> SNARAIARPTRSEYLARINEENRLKHEIQELTQALALEKQNTVTLVAQAQQQAKAKPIVRSQPEKSLESTDQNTLALNIQFYDPKQLLSSVNQSVSVPYFKLCQLFLNKSIELCTKHYHLKATDIDVVDEFHAE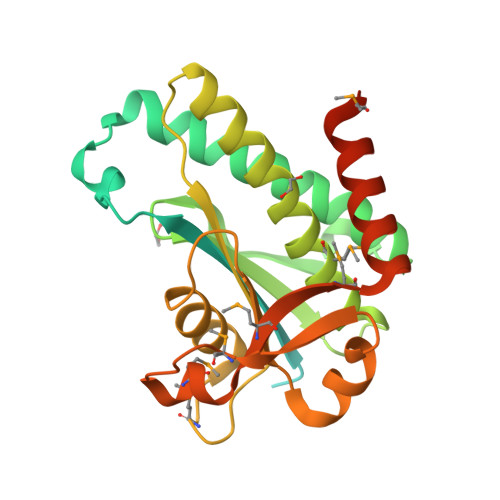GATLAISTSHPHAVECLLMVGTVFQLLSDVLYKRYREDKRFALQTRSAVCNAVEAMQIDAKEAAQRLAQHLHAKESALYLDNEQLKAIQDSYQLVAMPNPSNVMTRHAFMINGMNAECAELAQNIRTEILMGKKSIPQNDSPSSAAS2-[2-(3-chlorophenyl)ethyl]-1H-benzimidazol-7-ol | C15 H13 Cl N2 O 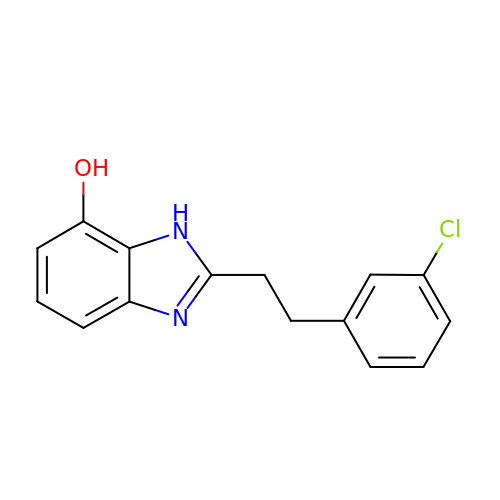| OTJBWWCEPHZWEI-UHFFFAOYSA-N>GPAVPRMVVLHSLLGMAVLIAIAVLLSTDRKAINIRTVAGAFLIQVALGALVLYVPQGRDMLGEASKTISNVIAYGNNGVDFLFGGLVSEKMFEVFGGGGFVFALRVLPMIVFFSSLMAVLYYIGVMQLLIKVIGGFLQKMLGTSKAESMSAAASIFVGQTEAPLVVRPYIRRMTESELFAVMSGGLASVAGSVLAGYVQMGVPLPYLIAASFMAAPGGLLFAKLLVPETERTQNDAEVLAENEDEKPTNVIDAAASGAVTGAQIAIAVGASLLAFVALIAMINGIIGGVGGWFGHGDLTLQAILGWLFSPLAWVIGVPWSEAGIAGSLIGQKVVINEFVAYSEFVKYLKPEAAVQLSDTTKAIISFALCGAANLGSIAVLVGGLSIMAPKRRKDVARLGIKAVVAGSLSNLMSAVIAGL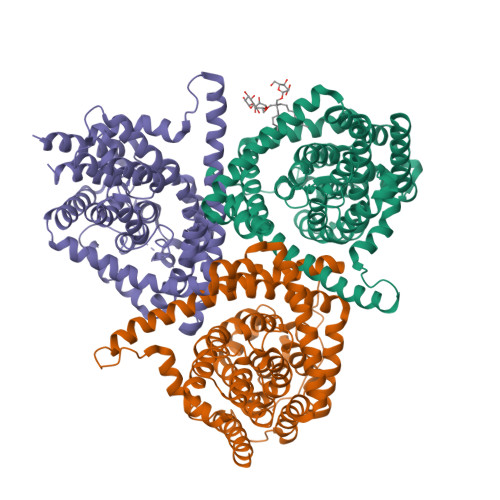FTGLSGASVLG[3x]>ATAAEIAALPRQKVELVDPPFVHAHSQVAEGGPKVVEFTMVIEEKKIVIDDAGTEVHAMAFNGTVPGPLMVVHQDDYLELTLINPETNTLMHNIDFHAATGALGGGGLTEINPGEKTILRFKATKPGVFVYHCAPPGMVPWHVVSGMNGAIMVLPREGLHDGKGKALTYDKIYYVGEQDFYVPRDENGKYKKYEAPGDAYEDTVKVMRTLTPTHVVFNGAVGALTGDKAMTAAVGEKVLIVHSQANRDTRPNLIGGHGDYVWATGKFNTPPDVDQETWFIPGGAAGAAFYTFQQPGIYAYVNHNLIEAFELGAAA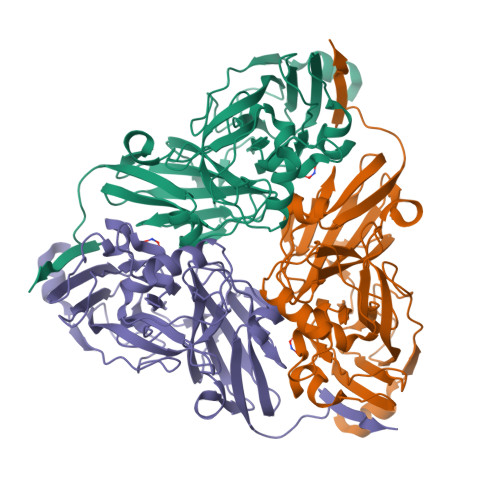HFKVTGEWNDDLMTSVLAPSGTIEGR[3x]> QDDSTPDSLFAGLVGEYYGTNSQLNNISDFRALVDSKEADATFEAANISYGRGSSDVAKGTHLQEFLGSDASTLSTDPGDNTDGGIYLQGYVYLEAGTYNFKVTADDGYEITINGNPVATVDNNQSVYTVTHASFTISESGYQAIDMIWWDQGGDYVFQPTLSADGGSTYFVLDSAILSSTGETPYTT

MpPA14 (Marinomonas primoryensis PA14 domain) lectin is a domain of a 1.5-MDa adhesin responsible for a symbiotic bacterium-diatom interaction in Antarctica. Bioinformatic analyses indicated the presence of an ∼20-kDa domain near the C terminus of MpIBP that is a member of the PA14 family, which is a carbohydrate-binding lectin module widely distributed across several kingdoms of life. PA14 domains share a β-sandwich fold and the presence of two consecutive aspartate residues in a cis peptide linkage (DcisD). The DcisD motif coordinates a Ca2+ ion that is directly involved in binding polar vicinal hydroxyl groups of various carbohydrates.

Similarly, 3-O-methyl-glucose cannot bind MpPA14 via the 3,4-diol because of the substituted methyl group on its C-3. This sugar compensates by binding using the 1,2-diol of the β-anomer, resulting in its considerably weaker binding to the lectin compared to that of glucopyranoses and mannose.The 22nd genetically encoded amino acid, pyrrolysine, plays a unique role in the key step in the growth of methanogens on mono-, di-, and tri-methylamines by activating the methyl group of these substrates for transfer to a corrinoid cofactor. A substrate:corrinoid methyltransferase catalyzes the demethylation of the specific methylamine, and subsequently transfers this methyl group onto an associated corrinoid protein. In summary, we have determined the structures of native MttB, and its complexes with a substrate analog, sulfite, and its physiological relevant corrinoid protein, MttC. These structures have provided new insights into the mechanism of activation of pyrrolysine that is distinct from the previously determined MtmB structure, and details of the key steps in the pyrrolysine-mediated transfer of methyl groups from methylamine substrates to the cobalamin cobalt in corrinoid proteins.

The 2.7 Å resolution structure of MttB-MttC complex was determined from crystals belonging to space group P21 with one full MttB hexamer bound to six MttC monomers with approximate D3 symmetry in the asymmetric unit. The electron density of the cofactor is consistent with 5-hydroxybenzimidazolyl cobamide, the predominant form of corrinoid extractable from Methanosarcina spp. grown on methanol. The cofactor is most likely in the pentacoordinate Co(II) state, as one nitrogen of His107 binds to the cobalt. In the native state, the helical cap domain blocks the β-face of the corrinoid, but upon methyltransferase binding, the cap domain is shifted to expose the corrinoid cofactor so that it can participate in the methyltransferase reaction. A similar positioning of the cap domain away from the corrinoid cofactor is observed in the MttB-MttC complex. This positioning exposes the β-face of the corrinoid cofactor and allows it to bind to the cavity formed by the TIM-barrel of MttB, thereby placing it directly over the pyrrolysine amino acid. The interface between the cap domain along with loops of core domain of MttC and dimerization loop of MttB provide the primary interactions that stabilize the MttB-MttC complex. Several MttB residues appear to undergo a conformational change upon formation of the MttB-MttC complex. The most notable of these is Met249, which adopts a conformation that moves its side chain away from the pocket in a fashion that appears suitable for facilitating TMA binding to pyrrolysine and its subsequent positioning near the corrinoid cobalt.

>[6x]MAKNNAVAGFNALNGVELNLFTTDELKAIHYATMEVLMDPGIQVSDPEARQIFKENGCEVNEKTNVVKIPEYLVRKALQLAPSRFVLWGRDKKFNTVQECGGKVHWTCFGTGVKVCKYQDGKYVTVDSVEKDIADIAKLCDWAENIDYFSLPVSARDIAGQGAQDVHETLTPLANTAKHFHHIDPVGENVEYYRDIVKAYYGGDEEEARKKPIFSMLLCPTSPLELSVNACQVIIKGARFGIPVNVLSMAMSGGSSPVYLAGTLVTHNAEVLSGIVLAQLTVPGAKVWYGSSTTTFDLKKGTAPVGSPELGLISAAVAKLAQFYGLPSYVAGSOSDAKVPDDQAGHEKTMTTLLPALAGANTIYGAGMLELGMTFSMEQLVIDNDIFSMVKKAMQGIPVSEETLAVESIQKVGIGNNFLALKQTRQLVDYPSNPMLLDRHMFGDWAAAGSKDLATVAHEKVEDVLKNHQVTPIDADIFKDMQAIVDKADKAFRGMGGHHHHHH;>MANKEEIIAKAKEAITDFDDELAEEVANEALAAGIDPVELIEKGFTAGMEEVGEKFGQGELFLPHVLAAAEAMNSGIKVITPEMEKRKSQTKSLGTVAIGTIEGDIHSIGKDIVASMLNIAGFKVVDLGRDVPINTFVEKVKELKPQVVASSALMTTTMVNQIQIEEQLKEAGVRDQVKTMVGGAPVTQDWADKIGADIYGESANDAVAKVKAALNVGGHHHHH[6x]> MKITAVRTHLLEHRLDTPFESASMRFDRRAHVLVEIECDDGTVGWGECLGPARPNAAVVQAYSGWLIGQDPRQTEKIWAVLYNALRDQGQRG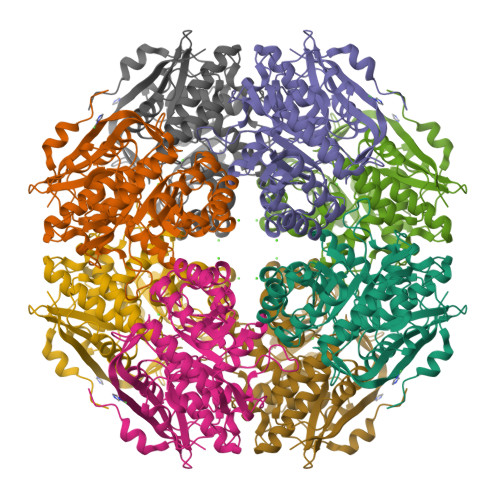LSLTALSGIDIALWDIKGKHYGASISMLLGGRWRESVRAYATGSFKRDNVDRVSDNASEMAERRAEGFHACKIKIGFGVEEDLRVIAAVREAIGPDMRLMIDANHGYTVTEAITLGDRAAGFGIDWFEEPVVPEQLDAYARVRAGQPIPVAGGETWHGRYGMWQALSAGAVDILQPDLCGCGGFSEIQKIATLATLHGVRIVPHVWGTGVQIAAALQFMAAMTPDPVRVNPIEPIMEFDRTHNPFRQAVLREPLEAVNGVVTIPDGPGLGIEINRDALTEFRMPDP>[6x]MGSDKIHHHHHHMIQSYPVERSRTIQTRLVLPPDTNHLGTIFGGKVLAYIDEIAALTAMKHANSAVVTASID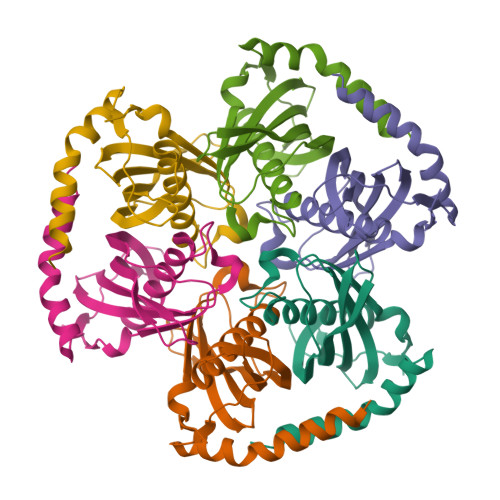SVDFKSSATVGDALELEGFVTHTGRTSMEVYVRVHSNNLLTGERTLTTESFLTMVAVDESGKPKPVPQVEPQTEEEKRLYETAPARKENRKKRAALR> MTKPSLISAKILQHINSIVWLQSKG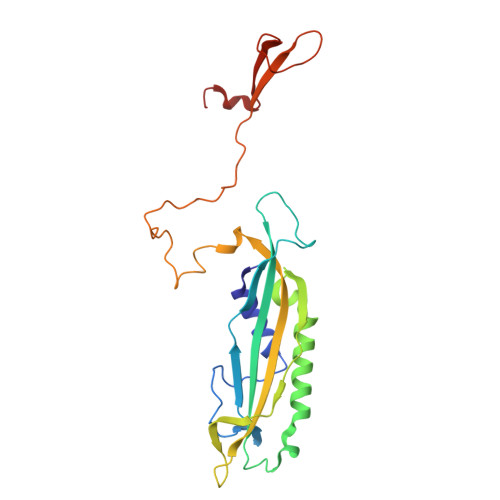IQEPLKPDVIVNNVAYPPNVIAEKPVTNIEVITNSSMIENTGGVRQFLCKAVFEYTIVWVFSREVYKTYHQIPRSQIQDLLVFCQQFVISAYQGIDPDITNIDLKPSQVLVKPTEDVNSDVSNSSSWSVVADLRFMIEFLTSLDEFLPIDFNKIQPPTWELLDDLDPIVPEQPFTLNGLIISLNKSELPKVRADESDTYQLEEILYIPPTIEDQI> FSEQTIPPSAKYGGRHTVTMIPGDGIGPELMLHVKSVFRHACVPVDFEEVHVSSNADEEDIRNAIMAIRRNRVALKGNIETNHNLPPSHKSRNNILRTSLDLYA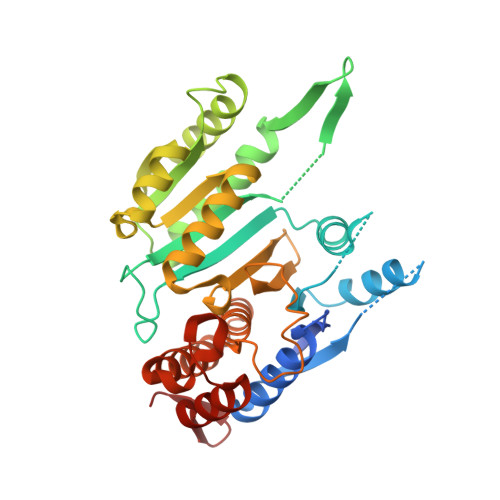NVIHCKSLPGVVTRHKDIDILIVRENTEGEYSSLEHESVAGVVESLKIITKAKSLRIAEYAFKLAQESGRKKVTAVHKANIMKLGDGLFLQCCREVAARYPQITFENMIVDNTTMQLVSRPQQFDVMVMPNLYGNIVNNVCAGLVGGPGLVAGANYGHVYAVFETATRNTGKSIANKNIANPTATLLASCMMLDHLKLHSYATSIRKAVLASMDNENMHTPDIGGQGTTSEAIQDVIRHIRVINGRAVEA>[2x]MGSSHHHHHHSQDLEVLFQGPHMAFEKPLRKLTFADLLQATNGFHNDSLIGSGGFGDVYKAILKDGSAVAIKKLIHVSGQGDREFMAEMETIGKIKHRNLVPLLGYCKVGDERLLVYEFMKYGSLEDVLHDPKKAGVKLNWSTRRKIAIGSARGLAFLHHNCSPHIIHRDMKSS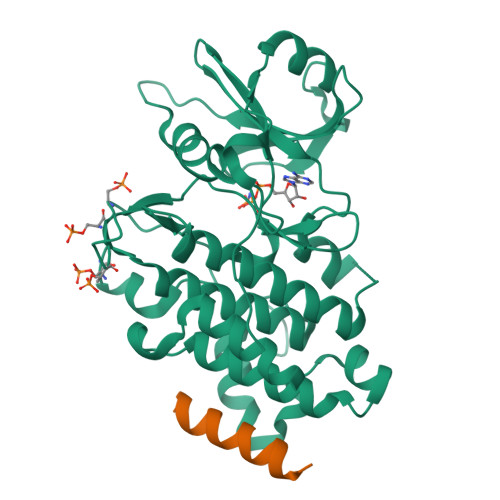NVLLDENLEARVSDFGMARLMSAMDTHLSVSTLAGTPGYVPPEYYQSFRCSTKGDVYSYGVVLLELLTGKRPTDSPDFGDNNLVGWVKQHAKLRISDVFDPELMKEDPALEIELLQHLKVAVACLDDRAWRRPTMVQVMAMFKEIQAGSGIDSQSTIRS;>STMEELQAAIQAAIAHCKNSY[2x]>MAQGMVTIYLPGEQQTLSVGPVENVAQLVTQPQLRDRLWWPGALLTDSAAKAKALKDYQHVMAQLASWEAEADDDVAATIKSVRQQLLNLNITGRLPVKLDPDFVRVDENSNPPLVGDYTLYTVQRPVTITLLGAVSGAGQLPWLAGRSVTDYLQDHPRLAGADKNNVMVITPEGETVVAPVALWNKRHVEPPPGSQLWLG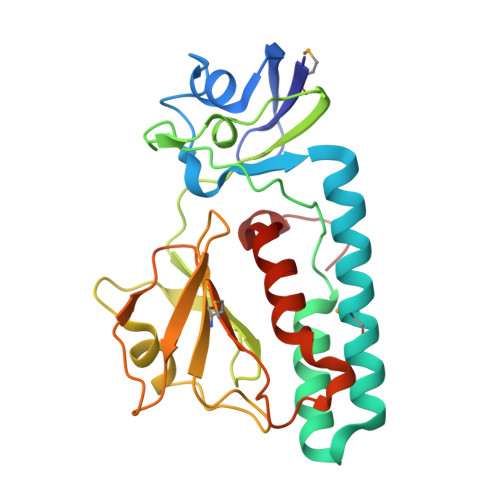FSAHVLPEKYADLNDQIVSVLTQRVPELEHHHHHH[4x]> MKFVSFNINGLRARPHQLEAIVEKHQPDVIGLQETKVHDDMFPLEEVAKLGYNVFYHGQKGHYGVA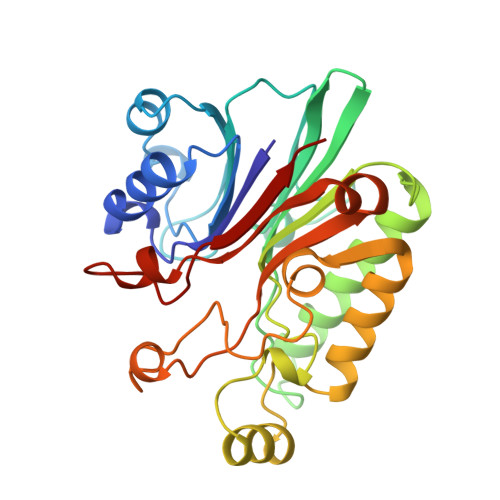LLTKETPIAVRRGFPGDDEEAQRRIIMAEIPSLLGNVTVINGYFPQGESRDHPIKFPAKAQFYQNLQNYLETELKRDNPVLIMGDMNISPTDLDIGIGEENRKRWLRTGKCSFLPEEREWMDRLMSWGLVDTFRHANPQTADRFSWFDYRSKGFDDNRGLRIDLLLASQPLAECCVETGIDYEIRSMEKPSDHAPVWATFRR>[2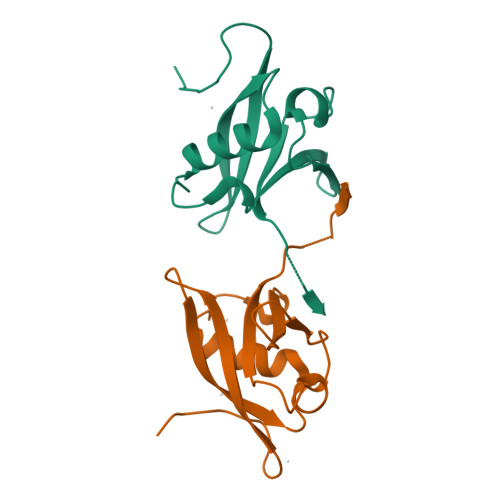x]MHHHHHHSSGRENLYFQGNQQVGDCCIIRVSLDVDNGNMYKSILVTSQDKAPAVIRKAMDKHNLEEEEPEDYELLQILSDDRKLKIPENANVFYAMNSTANYDFVLKKRTFTKGVKVKHGASSTLPRMKQKGLKIAKGIF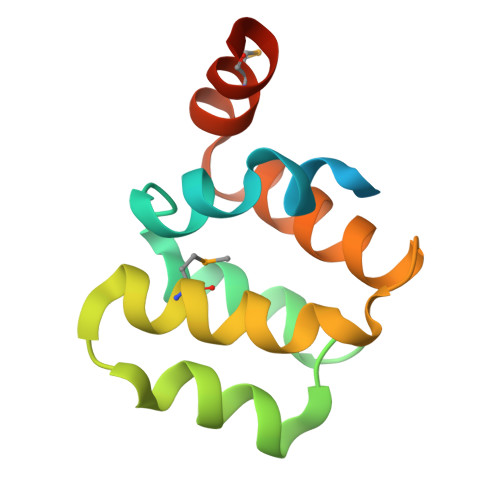> MGHHHHHHSHSPLDAPQLLHFVDQYREQLIARVTSVEVVLDKLHGQVLSQEQYERVLAENTRPSQMRKLFSLSQSWDRKCKDGLYQALKETHPHLIMELWEKGSKKG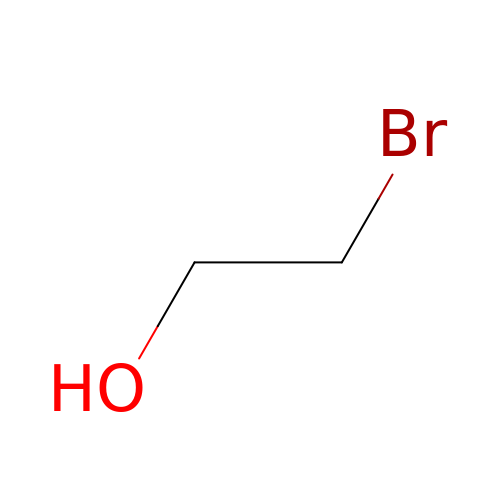2-BROMOETHANOL | C2 H5 Br O | LDLCZOVUSADOIV-UHFFFAOYSA-N>MGHHHHHHDDDKWERFLVPYRQAVEELKVKLKGIRTLYEYEDDHSPIEFVTGRVKPVASILEKARRKSIPLHEIETMQDIAGLRIMCQ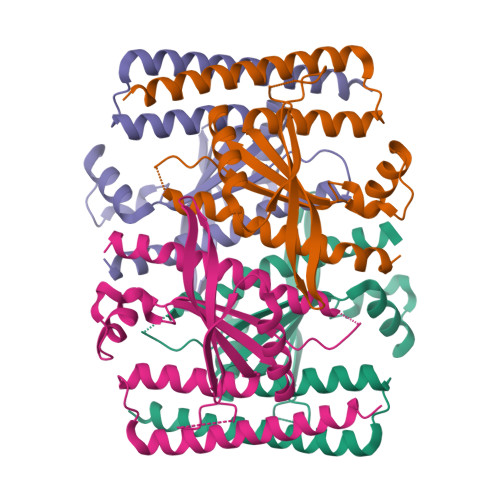FVDDIQIVKEMLFARKDFTVVDQRDYIAEHKESGYRSYHLVVLYPLQTVSGEKHVLVEIQIRTLAMNFWATIEHSLNYKYSGNIPEKVKLRLQRASEAASRLDEEMSEIRGEVQEAQAAFSRKKKGSEQQ[4x]> MRGSHHHHHHGMASMSVSTASTEMSVRKIAAHMKSNPNA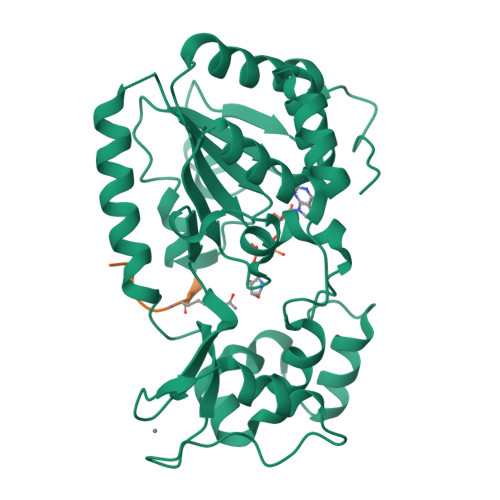KVIFMVGAGISTSCGIPDFRSPGTGLYHNLARLKLPYPEAVFDVDFFQSDPLPFYTLAKELYPGNFRPSKFHYLLKLFQDKDVLKRVYTQNIDTLERQAGVKDDLIIEAHGSFAHCHCIGCGKVYPPQVFKSKLAEHPIKDFVKCDVCGELVKPAIVFFGEDLPDSFSETWLNDSEWLREKITTSGKHPQQPLVIVVGTSLAVYPFASLPEEIPRKVKRVLCNLETVGDFKANKRPTDLIVHQYSDEFAEQLVEELGWQEDFEKILTAQ;> KGGAKRHRKILTAQ G-quadruplex (GQ) DNA is a well-studied non-canonical DNA structure formed by the π-π stacking of G-quartets. Here, we investigate the interaction of T1 with N-methyl mesoporphyrin IX (NMM), a water-soluble porphyrin with a distinctive central methyl group. Driven by this gap in knowledge, we determined crystal structures of T1-NMM and T7-NMM to 2.39 and 2.34 Å, respectively, as well as characterized stoichiometry, strength, and thermodynamic parameters of the T1-NMM interaction.

We designed the T7 construct to prevent the dimerization observed in T1 by adding 5’ and 3’ thymine overhangs. The T7-NMM crystal structure was solved in the P 63 space group to 2.34 Å and is characterized by an overall higher quality, so the subsequent discussion will be mainly focused on this structure. In both cases, the asymmetric unit contains two DNA chains, each of which binds one NMM molecule. Interestingly, the 5’ G-quartet–located at the dimer interface–has narrower grooves than the middle and 3’ G-quartets, 15.5 ± 0.2, 16.2 ± 0.2, and 16.6 ± 0.3 Å, respectively, in T7-NMM. T7 also contains 5’ and 3’ thymine overhangs with an average B-factor of 151.63 Å2. The flexibility of these terminal thymines may explain the destabilization of T7 with respect to T1 by -5.8 °C. The dimer in T7-NMM is further stabilized by base stacking between T5 and T′15 of chain B (where the prime (′) notation signifies a symmetry-related molecule). However, the T7 crystallographic dimer is likely an artifact of crystal packing, wherein the thymine overhangs–normally freely moving in solution and potentially inhibiting dimerization–are tucked into the grooves, thereby allowing the 5’ G-quartet to dimerize. T7, with two additional terminal thymines, also binds NMM with 1:1 stoichiometry, but with a lower Ka of 18 μM-1. We can explain the weaker binding of NMM to T7 (Ka of 18 μM-1) by the presence of terminal thymines that obstruct the binding surface at the 3’ G-quartet.

>TGGGTTGGGTTGGGTTGGGT[2x]>[6x]MKAVIFAYHDMGCQGVQAVLDAGY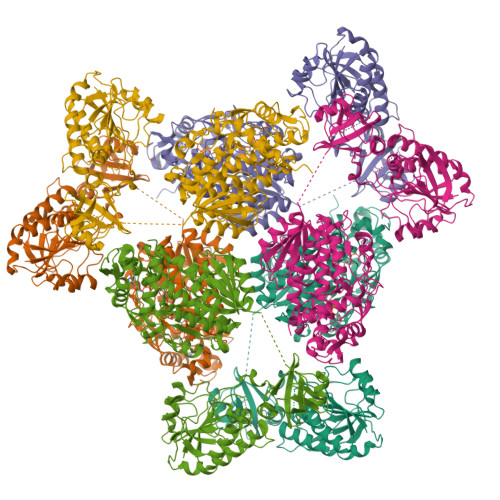EIAAIFTHADNPAENTFFGSVSRQAAELGIPVYAPDNVNHPIWVDRIAELAPDIIFSFYYRNLLSEEILHLAPAGAFNLHGSLLPAYRGRAPLNWVLVNGESETGVTLHRMVKRADAGEIVASQRVAIAQDDVALTLHHKLCQAARQLLNSILPTMKCGDIPSVPQRESDSTYYGRRRPEDGLIDWHKPVSTVHNLVRAVAAPWPGAFSYNGSQKFTIWSSRMCPDAQGALPGSVISVSPLRVACADGALEIITGQAGDDITVQGSQLAQTLGLVAGARLNRPPATSGKRRIRVLILGVNGFIGNHLTERLLNEENYEVYGMDIGSNAISRFLLHPRFHFVEGDISIHSEWIEYHVKKCDVVLPLVAIATPIEYTRNPLRVFELDFEENLRIIRYCVKYRKRVVFPSTSEVYGMCTDASFDEDKSNLIVGPVNKPRWIYSVSKQLLDRVIWAYGEKEGLRFTLFRPFNWMGPRLDSLNAARIGSSRAITQLILNLVEGTPIKLIDGGQQKRCFTDIRDGIEALFRIIVNDGDRCDGKIINIGNPDNEASIQELATLLLDSFDKHPLRCHFPPFAGFQVVESRSYYGKGYQDVAHRKPSIDNARRCLGWEPSIAMRDTVEETLDFFLRSVDIAERAS>MAIAQLATEYVFSDFLLKEPTEPKFKGLRLELAVDKMVTCIAVGLPLLLISLAFAQEISIGTQISCFSPSSFSWRQAAFVDSYCWAAVQQKNSLQSESGNLPLWLHKFFPYILLLFAILLYLPPLFWRFAAAPHICSDLKFIMEELDKVYNRAIKAAKSARDLDMRDGACSVPGVTENLGQSLWEVSESHFKYPIVEQYLKTKKNSNNLIIKYISCRLLTLIIILLACIYLGYYFSLSSLSDEFVCSIKSGILRNDSTVPDQFQCKLIAVGIFQLLSVINLVVYVLLAPVVVYT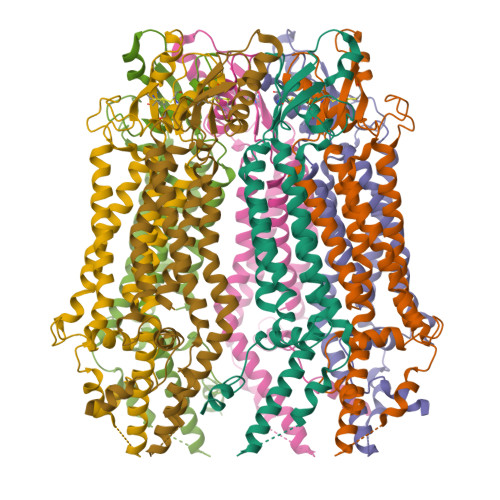LFVPFRQKTDVLKVYEILPTFDVLHFKSEGYNDLSLYNLFLEENISEVKSYKCLKVLENIKSSGQGIDPMLLLTNLGMIKMEVVEGKTPMSAEMREEQGNQTAELQGMNIDSETKANNGEKNARQRLLDSSCGSGSHHHHHHHHHH[7x]>[6x]GSHM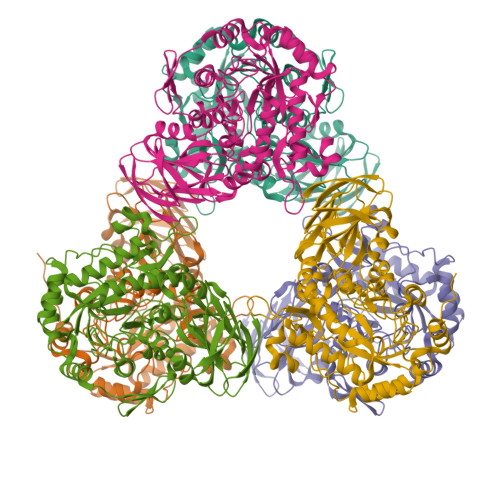RLNLGGAEVFLRAEGLEEAPGGVRLWGREVRVFPPFPAKGFFRHGWQSWSLAAWVDPAQAPTPLLPEARRPQADDPFLLEAGAWWGSGVGALRGPDGRALLLGALDLGARVLGREDLLLGRYAGKGGAWFLAYGPEEEVFAAYARLLPRRLSGRPPRVWCSWYSFYTRIGEDLLLRVLDEVAAFSFEVFQIDDGWQRALGDWEPNDRFPRGMAFLAERIRERGLRAGLWFAPFLVTADSPLFQKRPDWVLRDGEGRPVRAGFNWGRPLYALDAGNEEVVEWAADLVRKALAWGYDYLKLDFLYAAALPGAEGEARYRKAMARLREAAGEAYLLFCGAPVLASLGLADGLRVGPDVAPYWDNEERSFWLADPTGPGLRNALRSTLHRLWLMENVHVDPDVVYFRTRFNLLSPEEMRLQEALAHFTGFKATSDPPSWLLPEEKGRLEAFLAREVPVRRLGPYRFRVGEEEVDYAPLL> MASMTGGQQMGRGSMSRDPLPFFPPLYLGGPEITTENCEREPIHIPGSIQPHGALLTADGHSGEVLQMSLNAATFLGQEP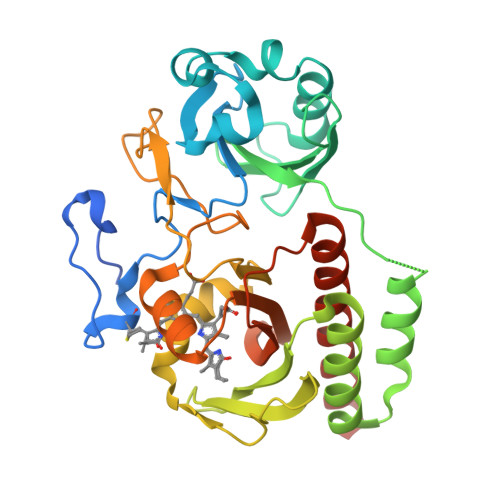TVLRGQTLAALLPEQWPALQAALPPGCPDALQYRATLDWPAAGHLSLTVHRVGELLILEFEPTEAWDSTGPHALRNAMSALESAPNLRALAEVATQTVRELTGFDRVMLYKFAPDATGEVIAEARREGLHAFLGHRFPASLIPAQARALYTRHLLRLTADTRAAAVPLDPVLNPQTNAPTPLGGAVLRATSPMHMQFLRNMGVGSSLSVSVVVGGQLWGLIACHHQTPYVLPPDLRTTLEYLGRELSEQVQVKEALEHHHHHH>MEKDLQLRVNEKLDVENILKDLDKYTPKRRGWTWRQPAENLQMGPFIYKDASTPLENSVALPSAKYFGDIDPQPLPVITTEIASGRFEDDIRRMRMAAWHGADHIMVIRTAGQSHYDGLIEGTPQGIGGVPITRKQVRAQRKALDLIEEEVGRPINYHSYVSGVAGPDIAVMFAEEGVNGAHQDPQYNVLYRNINMIRSFIDACESKTIMAWADMAQIDGAHNANATAREAWKVMPELMVQHALNSIFSLKVGMKKSNICLSTVPPTAPPAPSMYLDLPYAVALREMFEGYRMRAQMNTKYMEASTREATVTHVLNLLISKLTRADIQSTITPDEGRNVPWHIYNIEACDTAKQALIGMDGLMDMVQLKREGVLGDTVRELKERAVLFMEEIIEAGGYFNAVEQGFFVDSGYYPERNGDGIARQINGGIGAGTVFERDEDYMAPVTAHFGYNNVKQYDEALVSEPSKLIDGCTLEVPEKIVYIDELDENDNVNVRMEETKEFRHSSMIKPEVEWQADGTVLLTMFLPTSKR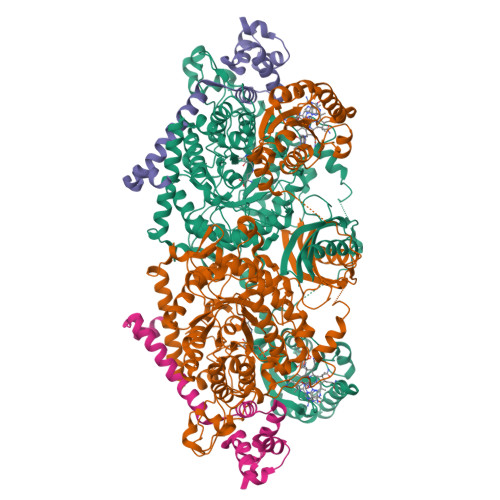VAEFAAIEFAKKMNLEEVEVINREVMQEAEGTRIELKGRVPFSIDINSLVIPPEPEILSEDEIREDIEKTPLKIVAATVGEDEHSVGLREVIDIKHGGIEKYGVEVHYLGTSVPVEKLVDAAIELKADAILASTIISHDDIHYKNMKRIHELAVEKGIRDKIMIGCGGTQVTPEVAVKQGVDAGFGRGSKGIHVATFLVKKRREMREGKSEDPNSSSVDKLAAALEHHHHHH[4x];>[4x]MKRADDFQQRRAHLANLSDEELQTRFWEMAEKIVDPLLDLGKKNTTPSIERSVLLRMGFSSLEAKAIVDKTMDRGLMGKGAGHIVYKIAKEKNISVREAGLALSEGKYWDDAIQIFKGGVK(4-oxoquinazolin-3(4H)-yl)acetic 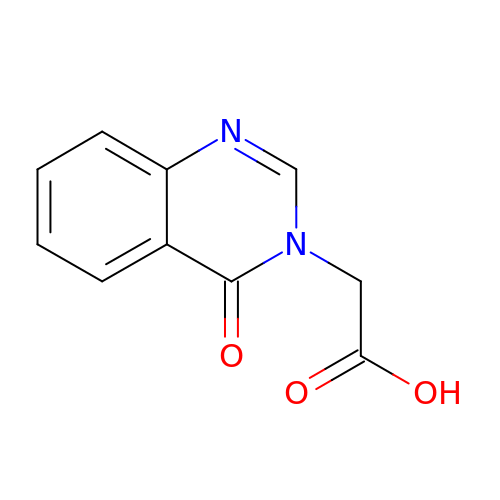acid | C10 H8 N2 O3 | BBBICQPTZBHLBM-UHFFFAOYSA-N> MAQGTLYIVSAPSGAGKSSLIQALLKTQPLYD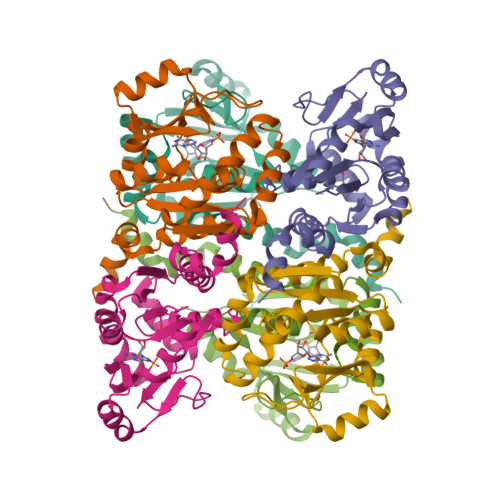TQVSVSHTTRQPRPGEVHGEHYFFVNHDEFKEMISRDAFLEHAEVFGNYYGTSREAIEQVLATGVDVFLDIDWQGAQQIRQKMPHARSIFILPPSKIELDRRLRGRGQDSEEVIAKRMAQAVAEMSHYAEYDYLIVNDDFDTALTDLKTIIRAERLRMSRQKQRHDALISKLLAD>[2x]GPHMKHPLMNVWTLWYLENDRSKSWEDMQNEITSFDTVEDFWSLYNHIKPPSEIKLGSDYSLFKKNIRPMWEDAANKQGGRWVITLNKS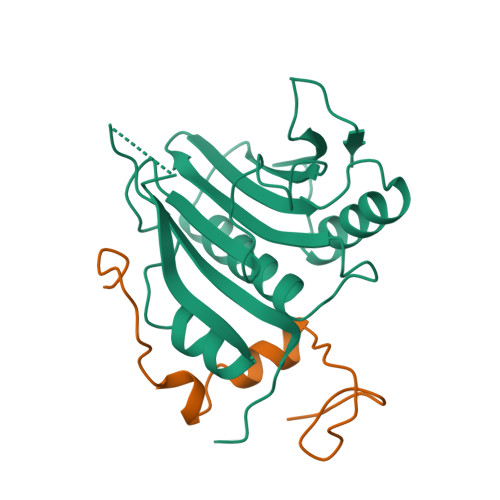SKTDLDNLWLDVLLCLIGEAFDHSDQICGAVINIRGKSNKISIWTADGNNEEAALEIGHKLRDALRLGRNNSLQYQLHKDTMVKQGSNVKSIYTL;>GPHMSIINYNEGQWSPNNPSGKKQYDREQLLQLREVKASRIQPEVKNVSILPQPNLMPSFIRNN[2x]> MSRSKRDNNFYSVEIGDSTFTVLKRYQNLKPIGSGAQGIVCAAYDAILERNVAIKKLSRPFQNQTHAKRAYRELVLMKVVNHKNIIGLLNVFTPQKSLEEFQDVYIVMELMDANLSQVIQMELDHERMSYL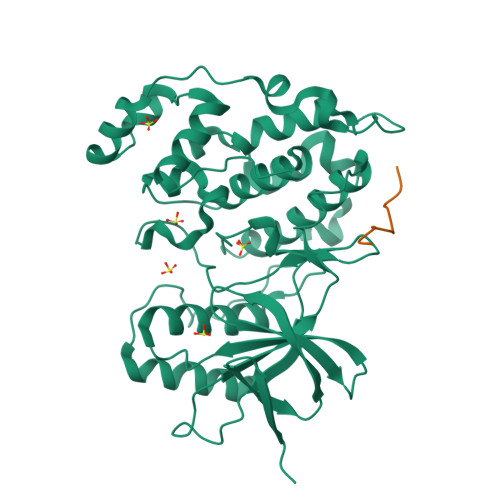LYQMLCGIKHLHSAGIIHRDLKPSNIVVKSDATLKILDFGLARTAGTSFMMTPYVVTRYYRAPEVILGMGYKENVDIWSVGCIMGEMIKGGVLFPGTDHIDQWNKVIEQLGTPSPEFMKKLQPTVRTYVENRPKYAGYSFEKLFPDVLFPADSEHNKLKASQARDLLSKMLVIDASKRISVDEALQHPYINVWYDPSEAEAPPPKIPDKQLDEREHTIEEWKELIYKEVMDLEHHHHHH;> RPKRPTTLNLF>MWVYRLKGTLEALDPILPGLFDGGARGLWEREGEVWAFFPAPVDLPYEGVWEEVGDEDWLEAWRRDLKPALAPPFVVLAPWHTWEGAEIPLVIEPGMAFGTGHAETTRLALKALARHLRPGDKVLDLGTGSGVLAIAAEKLGGKALGVDIDPMVLPQAEANAKRNGVRPRFLEGSLEAALPFGPFDLLVANLYAELHAALAPRYREALVPGGRALLTGILKD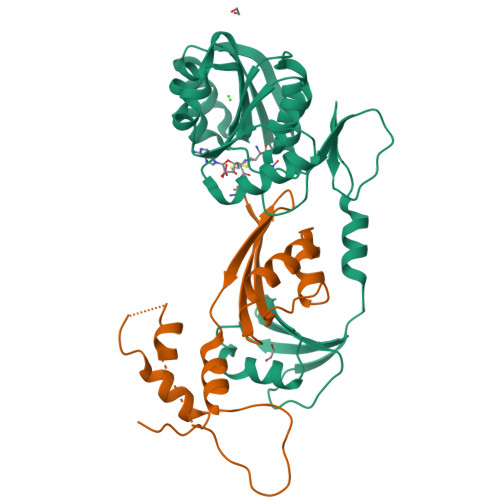RAPLVREAMAGAGFRPLEEAAEGEWVLLAYGR[8x];>MKKVVAVVKLQLPAGKATPAPPVGPALGQHGANIMEFVKAFNAATANMGDAIVPVEITIYADRSFTFVTKTPPASYLIRKAAGLEKGAHKPGREKVGRITWEQVLEIAKQKMPDLNTTDLEAAARMIAGSARSMGVEVVGAPEVKDA[8x]>[4x]MHHHHHHLPNITILATGGTIAGGGDSATKSNYTVGKVGVENLVNAVPQLKDIANVKGEQVVNIGSQDMNDNVWLTLAKKINTDCDKTDGFVITHGTTTMEETAYFLDLTVKCDKPVVMVGAMRPSTSMSADGPFNLYNAVVTAADKASANRGVLVVMNDTVLDGRDVTTTNTTDVATFK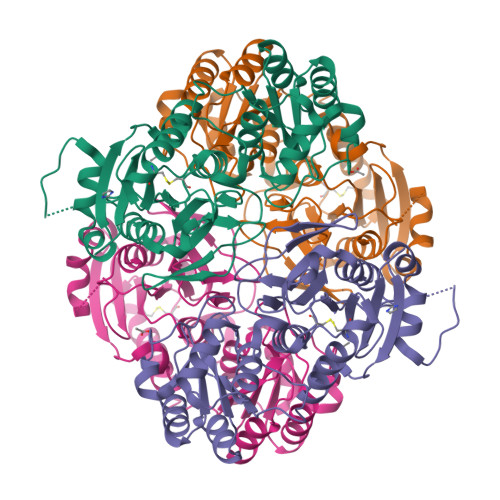SVNYGPLGYIHNGKIDYQRTPARKHTSDTPFDVSKLNELPKVGIVYNYANASDLPAKALVDAGYDGIVSAGVGNGNLYKSVFDTLATAAKTGTAVVRSSRVPTGATTQDAEVDDAKYGFVASGTLNPQKARVLLQLALTQTKDPQQIQQIFNQY> NETEVAKTSQDTTTASSSSEQNQSSNKTQTSAEVQTNAAAYWDGDYYVKDDGSKAQSEWIFDNYYKAWFYINSDGRYSQNEWHGNYYLKSGGYMAQNEWIYDSNYKSWFYLKSDGAYAHQEWQLIGNKWYYFKKWGYMAKSQWQGSYFLNGQGAMIQNEWLYDPAYSAYFYLKSDGTYANQEWQKVGGKWYYFKKWGYMARN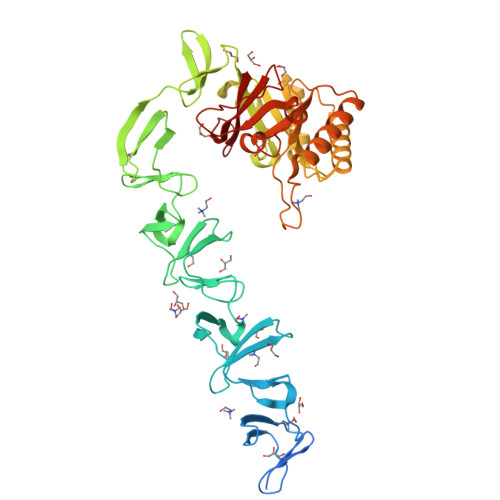EWQGNYYLTGSGAMATDEVIMDGARYIFAASGELKEKKDLNVGWVHRDGKRYFFNNREEQVGTEHAKKIIDISEHNGRINDWKKVIDENEVDGVIVRLGYSGKEDKELAHNIKELNRLGIPYGVYLYTYAENETDAENDAKQTIELIKKYNMNLSYPIYYDVQNWEYVNKSKRAPSDTDTWVKIINKYMDTMKQAGYQNVYVYSYRSLLQTRLKHPDILKHVNWVAAYTNALEWENPYYSGEKGWQYTSSEYMKGIQGRVDVSVWY> MHGLQDDPDLQALLKGSQLLKVKSSSWRRERFYKLQEDCKTIWQESRKVMRSPESQLFSIEDIQEVRMGHRTEGLEKFARDIPEDRCFSIVFKDQRNTLDLIAPSPADAQHWVQGLRKIIHHSGSMDQR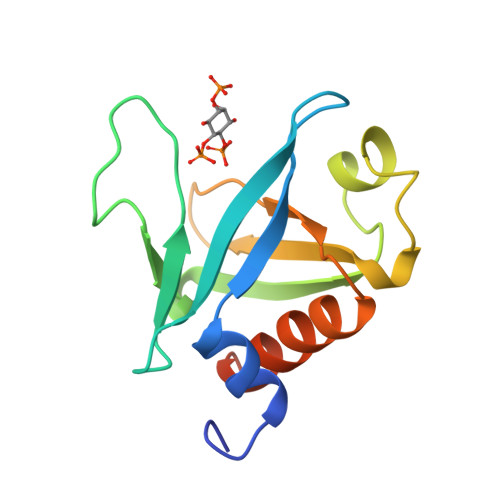QK>GAMSTTSTTIQVIGAGLPRTGTNSMKKALEIIYSKPCYHMYEIIFKKQSDISIWQQLIDETHKTTSDKRKIYNGLNELLNGYIATTDLPSCSFYKELMTMYPNAKVLLTIRDKYDWLYSLRKVVLPKSTDPWKLKIEEGDQVLGIDSNFYKMSEDSLKFAFQKNHINLDDDEILLECYDEYNRLVQEIVPPERLLIHHLGDGWESLCQFLNVDIPNGISYPCANSHHQMTQLTEQ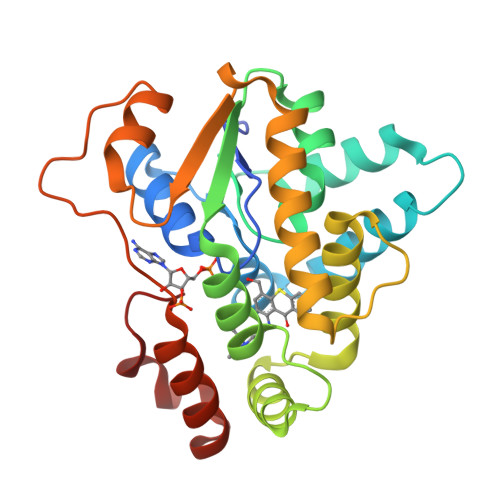LIKHKSLDDIIHMFPGLI[2x]> TVVNIDRINTKADGTIKVGGFKASLTTNAAHLNIGKGGVNLSNQASGRTLLVENLTGNITVDGPLRVNNQVGGYALAGSSANFEFKAGVDTKNGTATFNNDISLGRFVNLKVDAHTANFKGIDTGNGGFNTLDFSGVTNKVNINKLITASTNVAVKNFNINELIVKTNGVSVGEYTHFSEDIGSQSRINTVRLETGTRSIFSGGVKFKSGEKLVIDEFYYSP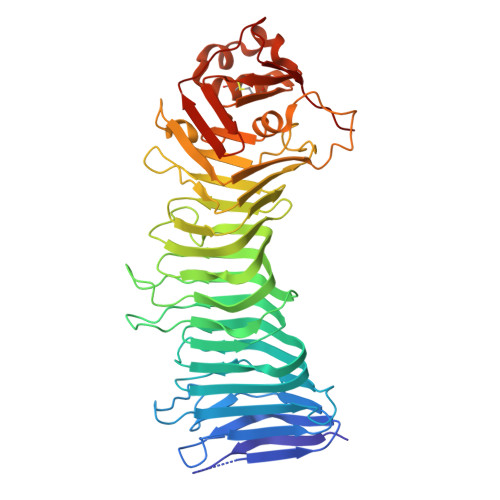WNYFDARNIKNVEITRKFASSTPENPWGTSKLMFNNLTLGQNAVMDYSQFSNLTIQGDFINNQGTINYLVRGGKVATLNVGNAAAMMFNNDIDSATGFYKPLIKINSAQDLIKNTEHVLLKAKIIGYGNVSTGTNGISNVNLEEQFKERLALYNNNNRMDTCVVRNTDDIKACGMAIGNQSMVNNPDNYKYLIGKAWKNIGISKTANGSKISVYYLGNSTPTENGGNTTNLPTNT> MGSSHHHHHHMFRTILVANRGEIALRVMRACRELGLRCVAVYSEADRDAPHVAYADDAFLIGPPSPAESYLNIDAIIRAAKATGAEAIHPGYGFLAENASFVRAVTAAGLIFIGPPAEAMERMGGKTAARREATAAGVPVVPGVLEPVTDAAEVRRLGKEFGYPIAIKAVGGGGGRGLRVVRSPEEVDEAFAAARREAEVAFKN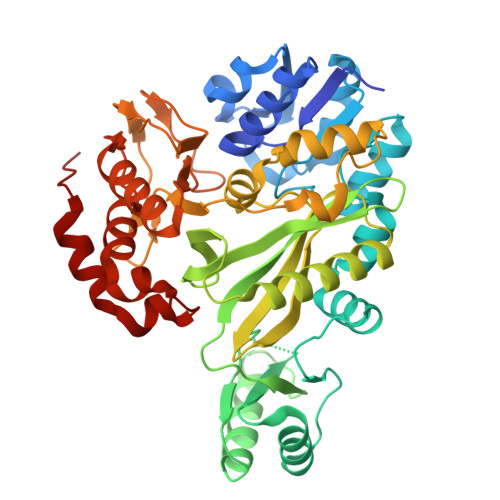GELYVEKYLDDPRHIEIQVLADRYGNAVALGERDCSVQRRHQKLIEECPSPALTPELRAEMGAAAVRLAKAVGYVSAGTLEFLFQDGRYYFLEMNTRIQVEHTVTEMVYGIDLVAAQIRIAQGEKLWFKQEDVVPRGHAIECRINAEDPLHNFRPALGTIGEYHEPVGFGVRVDSGVRAYYTVPSHYDSLLAKLITWGSDRQEAIARMRRALAEYRIEGVTTIIPFHQAALEHPVFTAGAATVNFIPRHPELFSRAAELTPPTAA> PGYTNMEKQAIARQYLWPKQVRESGMEGRIEVTDAAILRVISEYTREAGVRGLERELGKIARKG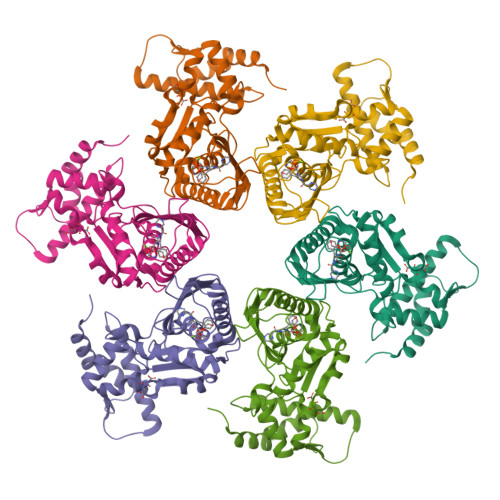AKFWLEGAWEGLRTIDASDIPTYLGIPRYRPDKAETEPQVGTAQGLAWTPVGGTLLTIEVAAVPGSGKLSLTGQLGEVMKESAQAALTYLRAHTQDYGLPEDFYNKVDLHVHVPDGATPKDGPSAGITMATAIASALSRRPARMDIAMTGEVSLRGKVMPIGGVKEKLLAAHQAGIHKIVLPKDNEAQLEELPKEVLEGLEIKLVEDVGEVLEYLLLPEPTMPPVVQPSDNRQQPGAGA> VTDQLEDLREHFKNTEEGKALVHHYEECAERVKIQQQQPGYADLEHKEDCVEEFFHLQHYLDTATAPRLF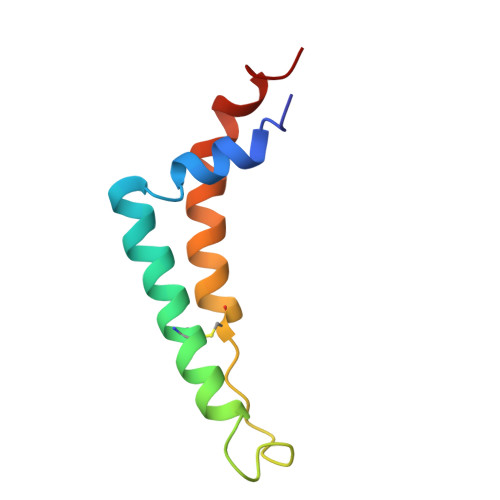DKLK2-DIMETHYLAMINO-ETHYL-DIPHOSPHATE | C4 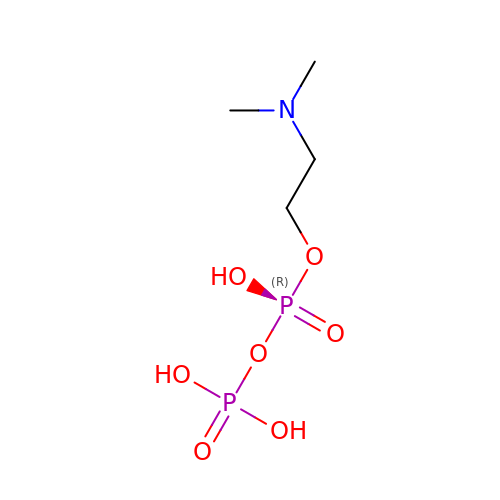H13 N O7 P2 | QGKJQRINUQGSJM-UHFFFAOYSA-N> A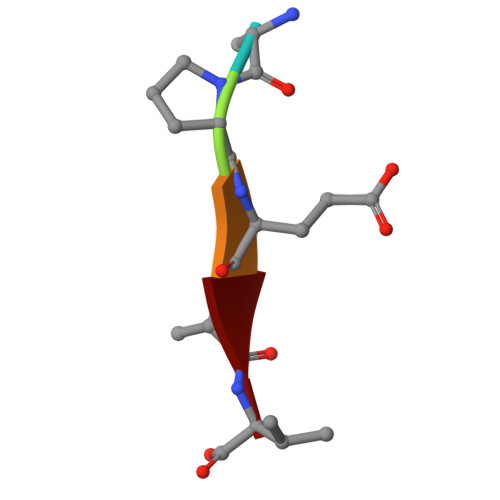PEAV>[4x]SVETIELKRGSNSVYVQYD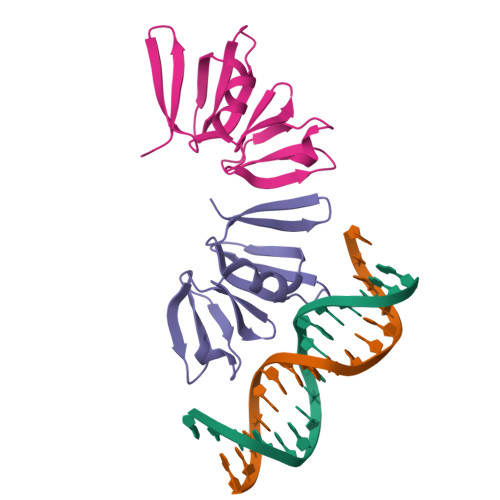DIMFFESSTKSHRLIAHLDNRQIEFYGNLKELSQLDDRFFRCHNSFVVNRHNIESIDSKERIVYFKNKEHCYASVRNVKKI> SNAMAKGVTIKDVAAEAGVSFKTVSNVINGTGSMRESTRGRVLEAMDKLNYTINLSARSLKTGTTGLLGLAIFDFSQPFASYLADQIIVCAREHHYGVIINTYGQNEHGLARAMRQANNLAADGWIVFADHAMGQHSKMLDQSYPLVLTGDWDAYGKVDQVTMPNVEAMRYTTNRLLDSGYRSIALFGADGSLGARHYRQATEGTQELRVQGYMQAYEEHGIEARMDMLFSGGLLTSDSGVRATNLMMDQGVRPDAIICLNDAMALGALHQLQVRGIRVPDDVQVVGFDNVPEATYAN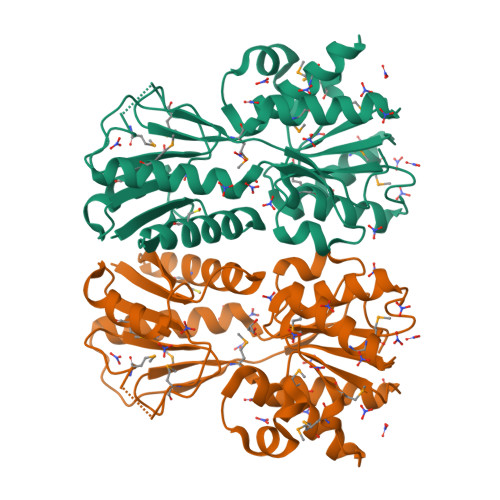PSLTTIDPHIDSYARHAVDMLIERIQGYDGAKRVYTSDFTLVERSSTSL> GHMGSSVLEELVQLVKDKNIDISIKYDPRKDSEVFANRVITDDIELLKKILAYFLPEDAILKGGHYDNQLQNGIKRVKEFLESSPNTQWELRAFM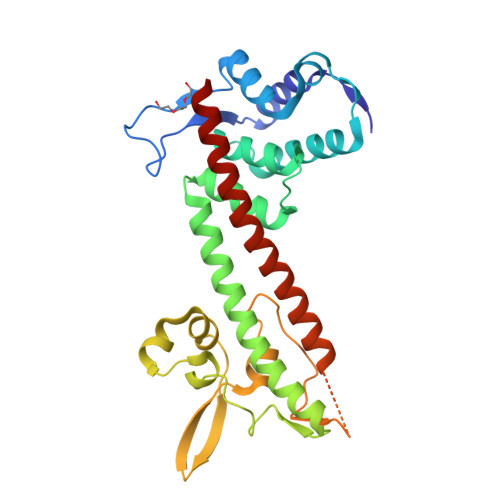AVMHFSLTADRIDDDILKVIVDSMNHHGDARSKLREELAELTAELKIYSVIQAEINKHLSSSGTINIHDKSINLMDKNLYGYTDEEIFKASAEYKILEKMPQTTIQVDGSEKKIVSIKDFLGSENKRTGALGNLKNSYSYNKDNNELSHFATTSSDKSRPLNDLVSQKTTQLSDITSRFNSAIEALNRFIQKYDSVMQRLLDD>GSSTNYGTIKWIFHALVFSYISFALISDKRYQKKEPLISSVHTKVKGIAEVKAEILENGMKKMVSGVFDTADYTFPLQGNSFFVMTNFIKTEGQQQGLCPDFPTARTICSSDRGCKKGRMDPQSKGIQTGRCVVYKERLKTCEVSAWCPIEEVKDAPRPALLNSAENFTVLIKNNIDFPGHNYTTRNILPGVNITCTFHKTQNPQCPIFRLGDIFQETGDSFSDVAIQGGIMGIEIYWDCNLDGWFHHCRPKYSFRRLDDKTTSESLYPGYNFRYAKYYKENNVEKRTLIKVFGIRFDILVFGTGGKFNVIQLAVYIGSVISYFGLATVFIDILINTYSASS[2x]

The P2X7 receptor, an extracellular ATP-gated ion channel predominantly expressed in immune cells of the blood and the brain, is an emerging target for treating refractory pain. P2X receptors are trimeric ligand-gated ion channels that facilitate extracellular-ATP mediated signaling along with the G protein-coupled P2Y receptors. For instance, the P2X7 receptor requires an unusually high concentration of ATP (EC50 ≥ 1 mM under physiological ion concentrations) for initial activation, its channel activity is facilitated by prolonged or repeated ATP applications, and it opens a membrane pore large enough for molecules up to ~900 Da to permeate. Here we identified and mapped the binding site for the P2X7 specific inhibitors for the first time using X-ray crystallography, and demonstrated by electrophysiological experiments that those inhibitors allosterically abrogate conformational changes associated with P2X7 receptor activation.

To confirm that allosterically-bound P2X7 inhibitors prevent the turret from narrowing upon ATP-binding, we obtained the crystal structure of the P2X7 receptor in the presence of both ATP and A804598. Consistent with the activation mechanisms proposed for P2X3 and P2X4, ATP-binding brings the dorsal fin domain towards the head domain and pushes the left flipper domain away from the ATP-binding pocket. These movements are coupled with widening of the lower body domain, though to an extent in which the transmembrane helices remain closed. In contrast, little conformational change was observed for the upper body domain including the turret and the drug-binding pockets, supporting that the turret closure is essential for P2X7 channel opening. Altogether, our data suggest that P2X7 receptors undergo unique conformational rearrangements where both the drug-binding pocket and the turret in the P2X7 receptor narrow upon ATP-binding. Although the lower body domain in our ATP/A804598-bound structure does seem to widen to some extent upon ATP-binding, the turret diameter remains locked due to A804598 binding, rendering the accompanying movement of the pore-lining transmembrane helices insufficient for channel opening. Closure of the turret, therefore, seems to be a prerequisite for full-widening of the lower body domain, which is necessary for channel opening.>[4x]MGSSHHHHHHSQDPMLNSFKLSLQYILPKLWLTRLAGWGASKRAGWLTKLVI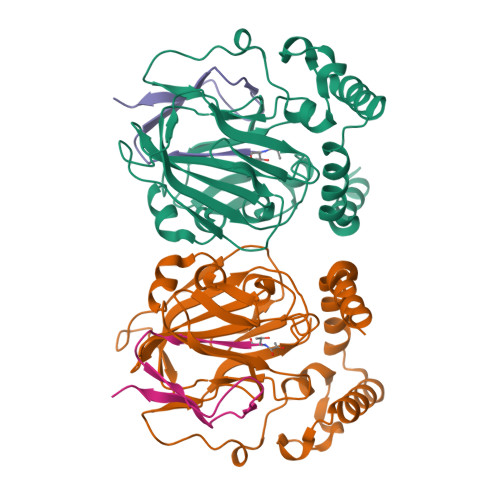DLFVKYYKVDMKEAQKPDTASYRTFNEFFVRPLRDEVRPIDTDPNVLVMPADGVISQLGKIEEDKILQAKGHNYSLEALLAGNYLMADLFRNGTFVTTYLSPRDYHRVHMPCNGILREMIYVPGDLFSVNHLTAQNVPNLFARNERVICLFDTEFGPMAQILVGATIVGSIETVWAGTITPPREGIIKRWTWPAGENDGSVALLKGQEMGRFKLG;>[4x]XTVINLFAPGKVNLVEQLESLSVTKIGQPLAVSTET> SSQIRQNYSTEVEAAVNRLVNLYLRASYTYLSLGFYFDRDDVALEGVCHFFRELAEEKREGAERLLKMQNQRGGRALFQDLQKPSQDEWGTTLDAMKAAIVLEKSLNQALLDLHALGSAQADPHLCDFLESHFLDEEVKLIKKMGDHLTNIQRLVGSQAGLGEYLFEHCTLKHD

Ferritin is a self-assembly protein cage consisting of 24 subunits with an 8 nm interior cavity. The 4-fold channel is composed of four E-helices forming a parallel four-helix bundle with C4 symmetry. Herein, we have engineered and constructed a gold clustering site at the 4-fold symmetric axis channel of the apo-ferritin cage. Using a series of X-ray crystal structures, we evaluated the stepwise accumulation process of Au ions into the cage and the formation of a multinuclear Au cluster in our designed cavity.

Thus, in our design, four L169Cs were expected as the main fixing residues and four R168Hs as auxiliary coordinating residues, which yielded the mutant design of apo-R168H/L169C-rHLFr. The apo-R168H/L169C-rHLFr mutant was expressed in E.coli and purified following the same procedure in our previous report. The resolution of apo-R168H/L169C-rHLFr is 1.5 Å. The mutation of R168H/L169C has a negligible effect on the conformation of the whole cage. The binding positions of Au ions were assigned by anomalous electron-density maps at 4σ and distinguished from Cd by comparison with the control apo-R168H/L169C-rHLFr structure and anomalous scattering at multiple wavelengths of 1.15 Å and 1.00 Å.> MGNYLEDCATVDVQARPTAYALAISSLGEFNSLTGGTSTDPVAEGNDYYYRFEIRAWEGSSGPQTNVTLNVTRTLGNSTFAGSGTKGVDFEVELDPDGPFGPASYAPVLSADVQVLAWG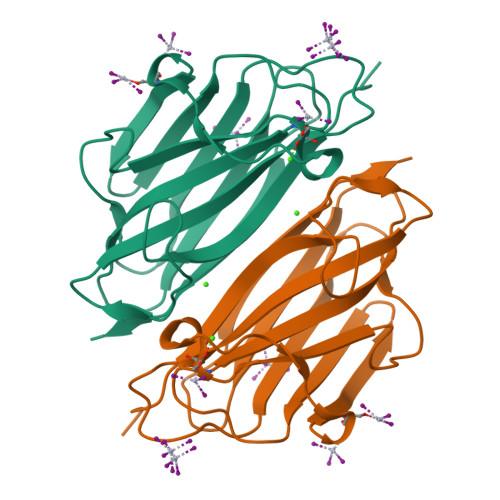PTGVQLRYLPSLAPGATLRFSLRANAVNGTNTTVQADATSTEAPGPYTVFETTTIIP> EQARPADDALAALGAQLFVDPALSRNATQSCATCHDPARAFTDPREGKAGLAVSVGDDGQSHGDRNTPTLGYAALVPAFHRDANGKYKGGQFWDGRADDLKQQAGQVMLNPVEMAMPDRAAVAARLRDDPAYRTGFEALFGKGVLDDPERAFDAAAEALAAYQATGEFSPFDSKYDRVMRGEEKFTPLEEFGYTVFITWNCRLCHMQRKQGVAERETFTNFEYHNIGLPVNETAREASGLGADHVDHGLLARPGIEDPA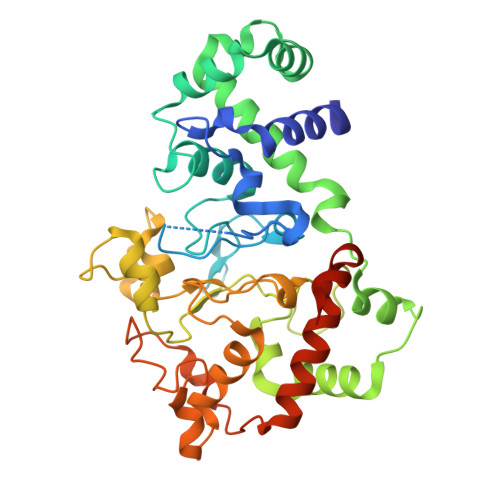QSGRFKVPSLRNVAVTGPYMHNGVFTDLRTAILFYNKYTSRRPEAKINPETGAPWGEPEVARNLSLAELQSGLMLDDGRVDALVAFLETLTDRRYEPLLEESRAAQKDHHHHHH> MSDPTQPAVPDFETRDPNSPAFWDERFERRFTPWDQAGVPAAF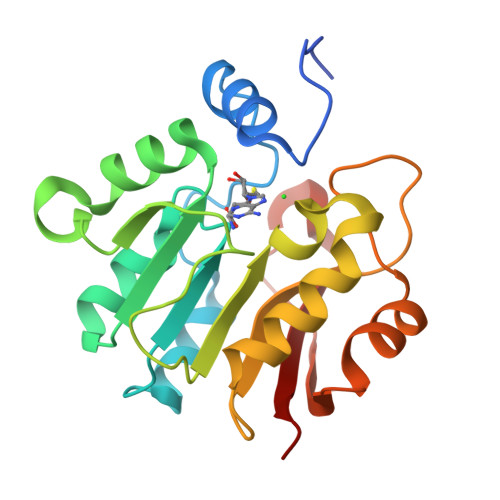QSFAARHSGAAVLIPGCGSAYEAVWLAGQGNPVRAIDFSPAAVAAAHEQLGAQHAQLVEQADFFTYEPPFTPAWIYERAFLCALPLARRADYAHRMADLLPGGALLAGFFFLGATPKGPPFGIERAELDALLTPYFDLIEDEAVHDSIAVFAGRERWLTWRRRA>[2x]TPVSEKQLAEVVANTITPLMKAQSVPGMAVAVIYQGKPHYYTFGKADIAANKPVTPQTLFELGSISKTFTGVLGGDAIARGEISLDDAVTRYWPQLTGKQWQGIRMLDLATYTAGGLPLQVPDEVTDNASLLRFYQNWQPQWK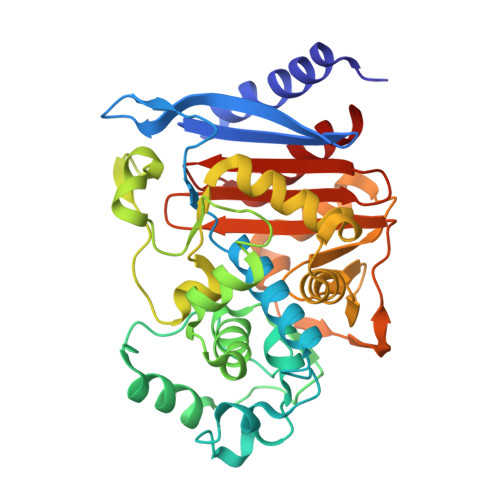PGTTRLYANASIGLFGALAVKPSGMPYEQAMTTRVLKPLKLDHTWINVPKAEEAHYAWGYRDGKAVRVSPGMLDAQAYGVKTNVQDMANWVMANMAPENVADASLKQGIALAQSRYWRIGSMYQGLGWEMLNWPVEANTVVEGSDSKVALAPLPVAEVNPPAPPVKASWVHKTGSTGGFGSYVAFIPEKQIGIVMLANTSYPNPARVEAAYHILEALQ>[2x]MATVENFNELPAHVWPRNAVRQEDGVVTVAGVPL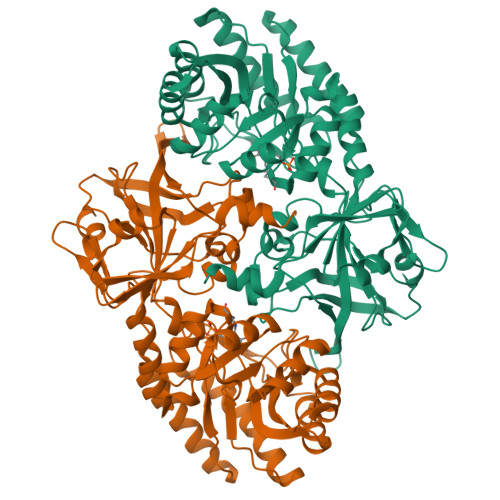PDLAEEYGTPLFVVDEDDFRSRCRDMATAFGGPGNVHYASKAFLTKTIARWVDEEGLALDIASINELGIALAAGFPASRITAHGNNKGVEFLRALVQNGVGHVVLDSAQELELLDYVAAGEGKIQDVLIRVKPGIEAHTHEFIATSHEDQKFGFSLASGSAFEAAKAANNAENLNLVGLHCHVGSQVFDAEGFKLAAERVLGLYSQIHSELGVALPELDLGGGYGIAYTAAEEPLNVAEVASDLLTAVGKMAAELGIDAPTVLVEPGRAIAGPSTVTIYEVGTTKDVHVDDDKTRRYIAVDGGMSDNIRPALYGSEYDARVVSRFAEGDPVSTRIVGSHCESGDILINDEIYPSDITSGDFLALAATGAYCYAMSSRYNAFTRPAVVSVRAGSSRLMLRRETLDDILSLEALEHHHHHH> GPTGMGNRGMEDLIPLVNRLQDAFSAIGQNADLDLPQIAVVGGQSAGASSVLENFVGRDFLPRGSGIVTRRPLVLQLVNATTEYAEFLHCKGKKFTDFEEVRLEIEAETDRVTGTNKGISPVPINLRVYSPHVLNLTLVDLPGMTKVPVGDQPPDIEFQIRDMLMQFVTKENCLILAVSPANSDLANSDALKVAKEVDPQGQRTIGVITKLDLMDEGTDARDVLENKLLPLRRGYIGVVNRSQKDIDGKKDITAALAAERKFFLSHPSYRHLADRMGTPYLQKVLNQQLTNHIRDTLPGLRNKLQSQLLSIEKEVEEYKNFRPDDPARKTKALLQMVQQFAVDFEKRIEGSGDQIDTYELSGGARINRIFHERFPFELVKMEFDEKELRREISYAIKNIHGIRTGLFTPDMAFETIVKKQVKKIREPCLKCVDMVISELISTVRQCTKKLQQYPRLREEMERIVTTHIREREGRTKEQVMLLIDIELAYMNTNHEDFIGFANAQQRSNQMNKKKTSGNQDEILVIRKGWLTINNIGIMKGGSKEYWFVLTAENLSWYKDDEEKEKKYMLSVDNLKLRDVEKGFMSSKHIFALFNTEQRNVYKDYRQLELACETQEEVDSWKASFLRAGVYPERVGDKEKASETEENGSDSFMHSMDPQLERQVETIRN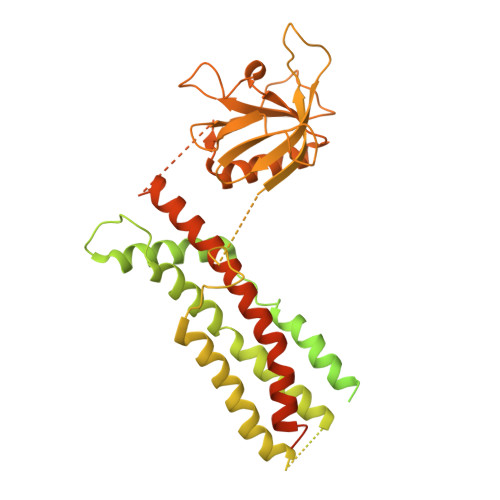LVDSYMAIVNKTVRDLMPKTIMHLMINNTKEFIFSELLANLYSCGDQNTLMEESAEQAQRRDEMLRMYHALKEALSIIGNINTTTV>MGQGPELHLASQFVNEACRALVFGGCVEKSSVSRNPEVPFESSAYRISASARGKELRLILSPLPGAQPQQEPLALVFRFGMSGSFQLVPREELPRHAHLRFYTAPPGPRLALCFVDIRRFGRWDLGGKWQPGRGPCVLQEYQQFRENVLRNLADKAFDRPICEALLDQRFFNGIGNYLRAEILYRLKIPPFEKARSVLEALQQHRPSPELTLSQKIRTKLQNPDLLELCHSVPKEVVQLGGRGYGSESGEEDFAAFRAWLRCYGMPGMSSLQDRHGRTIWFQGDPGPLAPKGRKS[3x]

Human endonuclease VIII-like 1 (hNEIL1) is a bifunctional DNA glycosylase of the Fpg/Nei family, which catalyzes the removal of damaged bases and subsequent incision of the newly generated abasic sites. Unlike traditional enzymes which are commonly referred to as highly specific biocatalysts, one special feature for hNEIL1 is its unique capability to recognize a wide range of substrates, including formamidopyrimidines, hydantoin lesions, oxidized, and dihydro-modified pyrimidine bases, derived from all four canonical bases. Here, by integrating structural, computational, and biochemical investigations, we show that hNEIL1 uses a triage mechanism to achieve broad specificity and reduce futile repair of normal bases. This mechanism involves two mutually competing interaction states: an activated state that commits catalysis and BER, and a quarantine state that temporarily separates and prevents the flipped base from catalysis via auto-inhibition.

For a naturally existing hNEIL1 variant (R242)14 in complex with dsDNAs containing OHU, Sp1, or Gh, the damaged bases are in close contact with the guanidine group of R242. Such conformation of the lesion recognition loop resembles that in the hNEIL1-Tg structure, where the positively charged side chain of residue 242 is contiguous to the solvent-exposed flipped base while the aromatic residue Y244 is laid away from the active site (thus called “242-in” conformation). Noteworthy, across all these structures, we observed an unusually short distance (~3.0 Å) between an outwards heterocyclic nitrogen atom of the nucleobases and the terminal nitrogen atom of residue 242. While repulsion is expected for the two groups if both are fully protonated (i.e., an −NH group in the nucleobase and a positively charged side chain of residue 242), we previously showed in the hNEIL1–Tg complex that hNEIL1 utilizes a tautomerization-dependent mechanism to recognize the flipped base. In this mechanism, the base undergoes a keto-enol tautomerization event where the originally protonated heterocyclic nitrogen atom becomes a hydrogen bond acceptor and hence can be hydrogen-bonded to residue 242. The fact that different recognition states were crystallographically captured for the same edited hNEIL1(R242) variant bound to different base lesions suggests that the flipped nucleobase per se also contributes to the stability of the interaction states. hNEIL1 repairs a diverse array of base damage, whose aromaticity and hydrophilicity differ greatly. Oxidized substrates of hNEIL1 are often bulky and contain non-planar structures; this disrupted aromaticity is expected to diminish the π–π stacking with Tyr244 and hence destabilize the quarantine state. Moreover, it is expected that the bases with less solvent interactions (e.g. DHU) would favor the formation of a stable quarantine state compared with the hydrophilic bases (Sp1, 5-OHU, Gh, and Tg).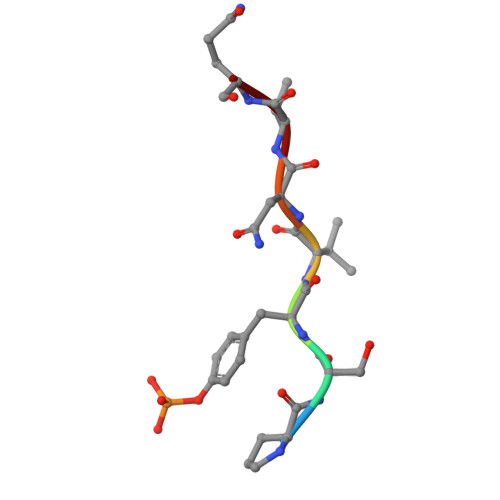> PSYVNVQ Pum is a founding member of the Pum/fem-3 mRNA-binding factor (FBF), or PUF family, of eukaryotic RBPs. Pum binds with high affinity to specific sequences in target mRNAs and represses protein expression and enhances mRNA degradation. Regulation of hb mRNA by Pum relies on the spatial distribution of Nos, a tandem CCHC Zn finger (ZF) RBP. Here, we report the crystal structures of Nos-Pum-RNA complexes, which reveal that Nos acts as a molecular clamp that embraces both Pum and RNA.

We determined a 3.7 Å crystal structure that reveals the molecular architecture of the Nos-Pum-RNA ternary complex. We crystalized Pum and Nos with a hb NRE2 RNA, 5´-AAAUUGUACAUAAGCC (the core PRE sequence is underlined, and we designate the first U of the core PRE as position +1 and number the four upstream nucleotides as −1 to −4). Strikingly, the structure illustrates how the Nos tandem ZFs envelop the RNA bases immediately upstream of the PRE and, together with the C-terminal region, embrace both the RNA and Pum. Comparison of the ternary and binary complexes reveals that the addition of Nos and the upstream nucleotides induces localized conformational changes in Pum that promote Nos-Pum interaction and binding of Pum to RNA upstream of the core PRE site. Loop residues between repeats R7 and R8 rearrange in the ternary complex to promote interaction of F1367Pum with the C-terminal α helix of Nos. In addition, the C-terminal α helix of Pum (helix α2 of repeat R8´) unfolds to promote interaction of residues with the upstream RNA backbone. The protein-protein interactions observed between Nos and Pum are focused between the C-terminal end of Nos (I376Nos to E385Nos) and the non-RNA-binding convex surface of Pum in repeats R7 and R8. For example, the side chain of Q1337Pum is within hydrogen bonding distance of main chain N and O atoms of I376Nos. The crystal structure of the Nos-Pum-hb RNA complex reveals that Nos binds to three nucleotides upstream of the core PRE when it joins the ternary complex, and we find that repression activity is highly sensitive to mutation of the interface. The first base upstream of the PRE, -1U, is inserted into a hydrophobic binding pocket formed by F321Nos, T366Nos, and Y369Nos (Figure 5A and Figure 2―figure supplement 1). The O4 atom of −1U is near the main chain N atom of T366Nos.

> SGRSRLLEDFRNQRYPNLQLRDLANHIVEFSQDQHGSRFIQQKLERATAAEKQMVFSEILAAAYSLMTDVFGNYVIQKFFEFGTPEQKNTLGMQVKGHVLQLALQMYGCRVIQKALESISPEQQQEIVHELDGHVLKCVKDQNGNHVVQKCIECVDPVALQFIINAFKGQVYSLSTHPYGCRVIQRILEHCTAEQTTPILDELHEHTEQLIQDQYGNYVIQHVLEHGKQEDKSILINSVRGKVLVLSQHKFASNVVEKCVTHATRGERTGLIDEVCTFNDNALHVMMKDQYANYVVQKMIDVSEPTQLKKLMTKIRPHMAALRKYTYGKHINAKLEK;> SRGASNSSNNNNNNNKVYKRYNSKAKEISRHCVFCENNNEPEAVINSHSVRDNFNRVLCPKLRTYVCPICGASGDSAHTIKYCPKKPIITMEDAIKAESFRLAKSSYYKQQMKV> SPSAEACGYSDRVAQLTLG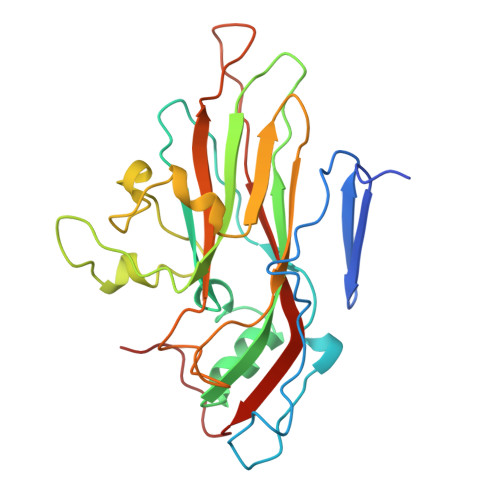NSTITTQEAANICVAYGCWPAKLSDTDATSVDKPTEPGVSADRFYTLRSKPWQADSKGWYWKLPDALNNTGMFGQNAQFHYIYRGGWAVHVQCNATKFHQGTLLVLAIPEHQIATQEQPAFDRTMPGSEGGTFQEPFWLEDGTSLGNSLIYPHQWINLRTNNSATLILPYVNAIPMDSAIRHSNWTLAIIPVAPLKYAAETTPLVPITVTIAPMETEYNGLRRAIASNQ> PGECSVNVIPKKNLDKAKFFSGTWYETHYLDMDPQATEKFCFSFAPRESGGTVKEALYHFNVDSKVSFYNTGTGPLESNGAKYTAKFNTVDKKGKEIKPADEKYSYTVTVIEAAKQSALIHICLQEDGKDIGDLYSVLNRNKNALPNKKIKKALNKVSLVLTKFVVTKDLDCKYDDKFLSSWQK

Here we report on seven crystal structures of NP7 at low and high pH and with different heme ligands. The overall fold of NP7 resembles that of other NPs. Eight anti-parallel β-strands (A to H) form a barrel that hosts the heme cofactor including the ligation by the proximal His60 residue. One of the most interesting features of NP7 is its ability to bind to negatively charged membranes.

However, no significant conformational differences were found between the X-ray structures collected at two different pHs (5.8 and 7.8; RMSD = 0.22 Å), even though this might simply arise from the packing of NP7 molecules in the crystal. Overall, these findings suggest that the ill-defined heme density of the unliganded NP7 reflects the movement of the cofactor inside the heme pocket according to the two coordination states. However, packing effects also explain the large structural similarity observed for the different ligand-bound and unbound structures, although such a structural similarity does not permit to rationalize the effect of deletion of the N-terminal residues on the binding affinities of certain ligands nor the pH sensitivity of NP7.> GPGSMPSKEASSRNLPISGRDTNGKTYRSTDEMWKAELTGDLYDPEKGWYGKALEYWRTVPATVSGVLGGMDHVHDVDIEGSRNFIASLPGHGTSRALDCGAGIGRITKNLLTKLYATTDLLEPVKHMLEEAKRELAGMPVGKFILASMETATLPPNTYDLIVIQWTAIYLTDADFVKFFKH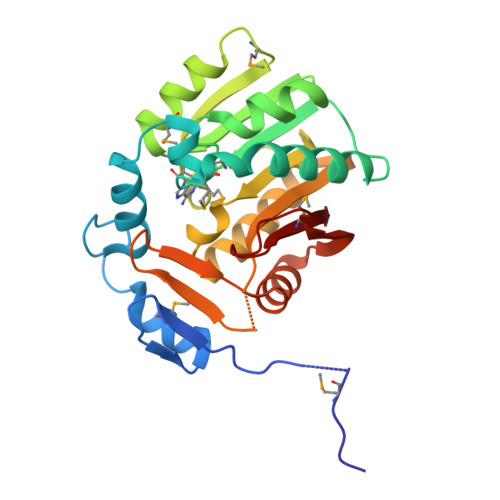CQQALTPNGYIFFKENCSTGDRFLVDKEDSSLTRSDIHYKRLFNESGVRVVKEAFQEEWPTDLFPLKMYALK Human soluble epoxide hydrolase (hsEH) is a cytosolic enzyme which modulates the metabolism of bioactive epoxy fatty acids (EpFAs), by converting them into their corresponding vicinal diols. In mammals, the enzyme is composed of two structurally distinct domains connected by a proline-rich linker. Whilst the N-terminal domain exerts phosphatase activity on glycerophospoholipids and lysophosphatidic acids, the hydrolytic activity on EpFAs resides in the C-terminal domain (CTD). This hydrolysis involves a SN2 nucleophilic attack by D335 on the least hindered carbon atom of the epoxide, followed by water-mediated release of the alkyl-enzyme intermediate, assisted by D496 and H524.

First, we solved the structure of apo hsEH CTD by X-ray crystallography, and our results were found to be in excellent agreement with previously deposited structures of the full-length enzyme, with an RMSD of 0.257 Å on all CTD heavy atoms. The apoprotein crystallised in space group I2, with two hsEH CTD molecules in the asymmetric unit forming a homodimer. Superposition of the apo and holo crystal structures gave an RMSD on all heavy atoms of 0.198 Å, indicating a high similarity of the two structures. Minor changes were observed in two regions proximal to the F267 Pocket.

>[2x]MHHHHHHSTENLYFQGSSTSCNPSDMSHGYVTVKPRVRLHFVELGSGPAVCLCHGFPESWYSWRYQIPALAQAGYRVLAMDMKGYGESSAPPEIEEYCMEVLCKEMVTFLDKLGLSQAVFIGHDWGGMLVWYMALFYPERVRAVASLNTPFIPANPNMSPLESIKANPVFDYQLYFQEPGVAEAELEQNLSRTFKSLFRASDESVLSMHKVCEAGGLFVNSPEEPSLSRMVTEEEIQFYVQQFKKSGFRGPLNWYRNMERNWKWACKSLGRKILIPALMVTAEKDFVLVPQMSQHMEDWIPHLKRGHIEDCGHWTQMDKPTEVNQILIKWLDSDARNPPVVSKM> XL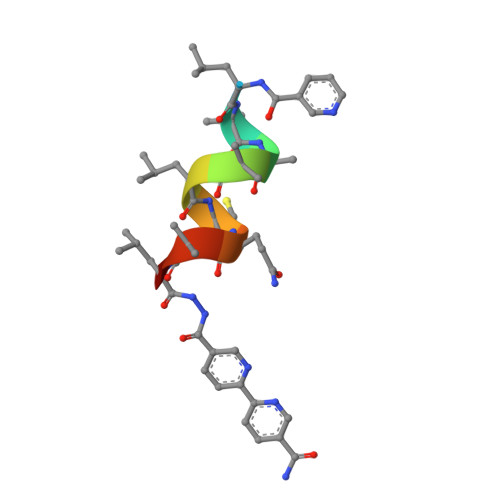AAALCQALX> MADSTTPGYTVVKNDWKKAVKQLQDGLKNKTISTIKVSFNGNSVGEVTPASSGAKKADRDAAAEKLYNLVNTQLDKLGDGDYVDFEVTYNLATQIITKAEAEAVLTKLQQYNDKVLINSATDTVKGMVSDTQVDSKNVAANPLKVSDMYTIPSAITGSDDSGYSIAKPTEKTTSLLYGTVGDATAGKAITVDTASNEAFAGNGKVIDYNKSFKATVQGDGTVKTSGV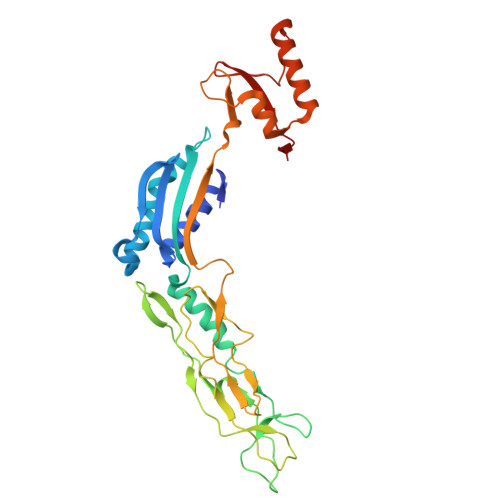VLKDASDMAATGTIKVRVTSAKEESIDVDSSSYISAENLAKKYVFNPKEVSEAYNAIVALQNDGIESDLVQLVNGKYQVIFYPEGKRLETKS> QIRYSVPEETDKGTVVGNISKDLGLEPRELAERGVRIVSRGRSQLFSLNPRGGSLVTAGRIDREELCAQSTPCLVNINILVEEKGKLFGVEIEITDINDNNPKFHVGDLEVKINEIAAPGARYPLPEAVDPDVGINSLQSYQLSPNRHFSLHLQTGDDGTINPELVLERTLDREEEPTHHLVLTASDGGEPRRSSTALIQITVLDTNDNAPVFDQPVYRVKVLENVAPGTLLLTVRASDPDEGVNGKVTYKFRKINEKQSLLFHLHENTGEMTVAKNLDYEECSLYEMEIQA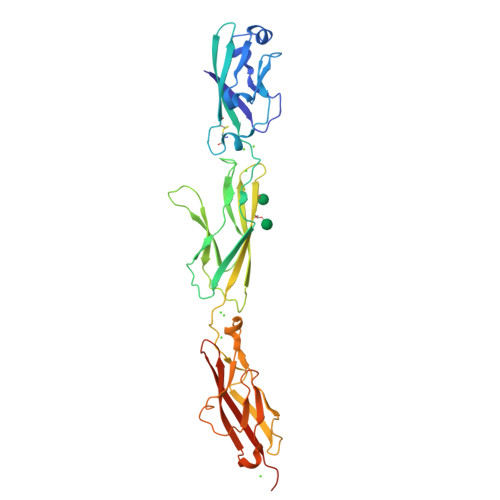EDVGALLGRSKVIIMVEDVNDHHHHHHHH>[2x]MNASEFRRRGKEMVDYVANYMEGIEGRQVYPDVEPGYLRPLIPAAAPQEPDTFEDIINDVEKIIMPGVTHWHSPYFF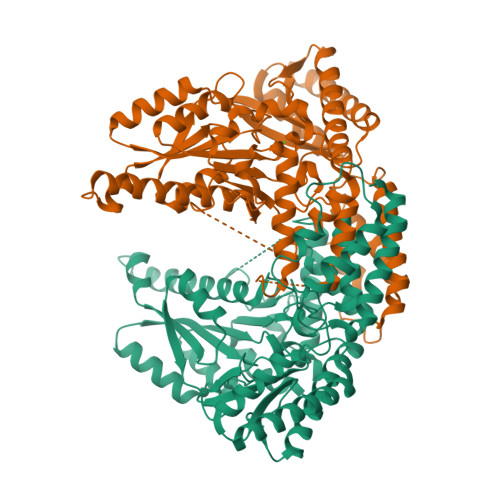AYFPTASSYPAMLADMLCGAIGCIGFSWAASPACTELETVMMDWLGKMLELPKAFLNEKAGEGGGVIQGSASEATLVALLAARTKVIHRLQAASPELTQAAIMEKLVAYSSDQAHSSVERAGLIGGVKLKAIPSDGNFAMRASALQEALERDKAAGLIPFFMVATLGTTTCCSFDNLLEVGPICNKEDIWLHVDAAYAGSAFICPEFRHLLNGVEFADSFNFNPHKWLLVNFDCSAMWVKKRTDLTGAFRLDPTYLKHSHQDSGLITDYRHWQIPLGRRFRSLKMWFVFRMYGVKGLQAYIRKHVQLSHEFESLVRQDPRFEICVEVILGLVCFRLKGSNKVNEALLQRINSAKKIHLVPCHLRDKFVLRFAICSRTVESAHVQRAWEHIKELAADVLRAERE>MSLKLYGFSVSNYYNMVKLALLEKGLTFEEVTFYGGQAPQALEVSPRGKVPVLETEHGFLSETSVILDYIEQTQGGKALLPADPFGQAKVRELLKEIELYIELPARTCYAESFFGMSVEPLIKEKARADLLAGFATLKRNGRFAPYVAGEQLTLADLMFCFSVDLANAVGKKVLNIDFLADFPQAKALLQLMGENPHMPRILADKEASMPAFMEMIRSGKREGHHH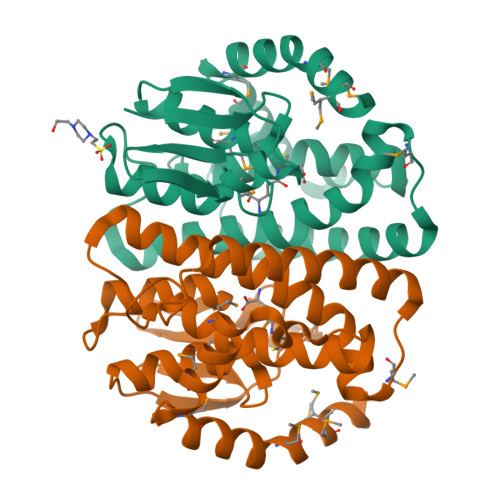HHH[4x]>GSGNAKLNTETPQSFVSNGSNTSFSAEDILAKAQQYAQEHELNFSGSLSPVDAWQLVQQGEAVLVDVRTNEERKFVGYVPESIHVAWATGTSFNRNPRFLKELESKVGKDKTILLLCRSGNRSTQAAEAAFNAGFEHIYNVL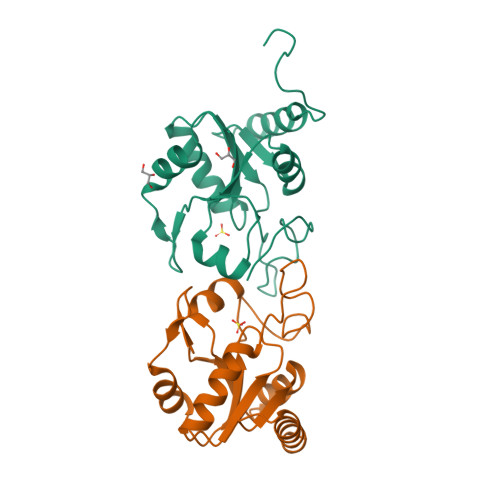EGFEGDLNEQQQRNQKNGWRIHQLPWQQD[2x]>GSAKDPMKQTLLLVEDDKNLADGLLVSLEQAGYECLHVERIADVEPQWKKADLVILERQLPDGDSVQHLPEWKKIKDVPVILLTALVTVKDKVAGLDSGANDYLTKPFAEAELFARIRAQLRA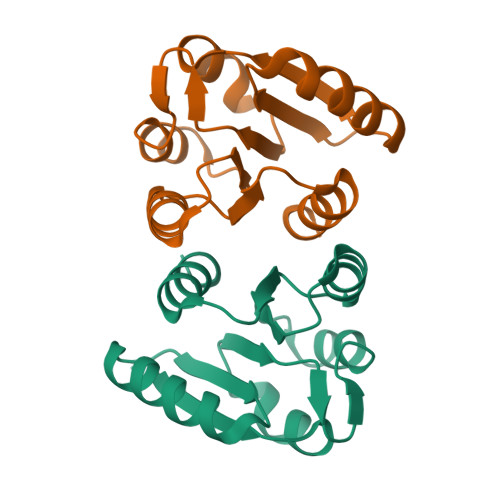PDS[2x]[2-[(3-chlorophenyl)methylamino]-7-methoxy-1,3-benzoxazol-5-yl]-(2,2-dimethylmorpholin-4-yl)methanone | C22 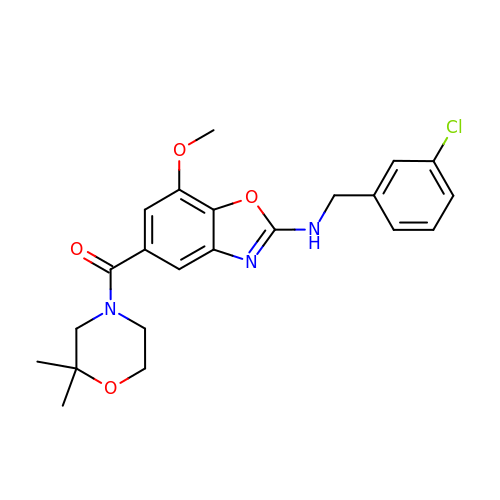H24 Cl N3 O4 | UZHJACGATLINFM-UHFFFAOYSA-N>[2x]MTERPRDCRPVVRRARTSDVPAIKQLVDTYAGKI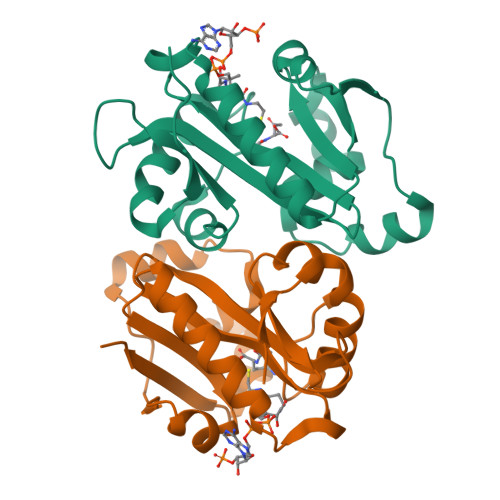LLEKNLVTLYEAVQEFWVAEHPDLYGKVVGCGALHVLWSDLGEIRTVAVDPAMTGHGIGHAIVDRLLQVARDLQLQRVFVLTFETEFFARHGFTEIEGTPVTAEVFDEMCRSYDIGVAEFLDLSYVKPNILGNSRMLLVLLEHHHHHH(1S)-1-(4-fluorophenyl)-2-(1H-imidazol-1-yl)ethyl 3,5-dichlorobenzoate | C18 H13 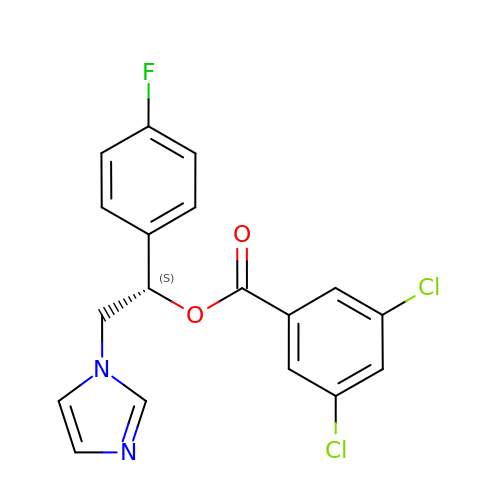Cl2 F N2 O2 | QANGFQMHUQHXKD-QGZVFWFLSA-N> GEVASVPLTNYLDSQYFGKIYLGTPPQEFTVLF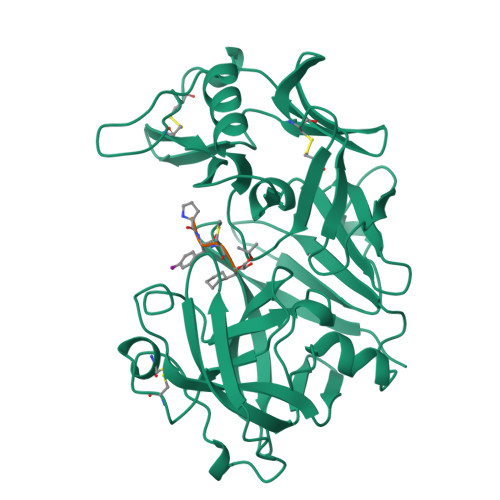DTGSSDFWVPSIYCKSNACKNHQRFDPRKSSTFQNLGKPLSIHYGTGSMQGILGYDTVTVSNIVDIQQTVGLSTQEPGDVFTYAEFDGILGMAYPSLASEYSIPVFDNMMNRHLVAQDLFSVYMDRNGQESMLTLGAIDPSYYTGSLHWVPVTVQQYWQFTVDSVTISGVVVACEGGCQAILDTGTSKLVGPSSDILNIQQAIGATQNQYGEFDIDCDNLSYMPTVVFEINGKMYPLTPSAYTSQDQGFCTSGFQSENHSQKWILGDVFIREYYSVFDRANNLVGLAKAI>MGVEDEPLLRENPRRFVIFPIEYHDIWQMYKKAEASFWTAEDVDLSKDIQHWESLKPEERYFISHVLAFFAASDGIVNENLVERFSQEVQITEARCFYGFQIAMENIHSEMYSLLIDTY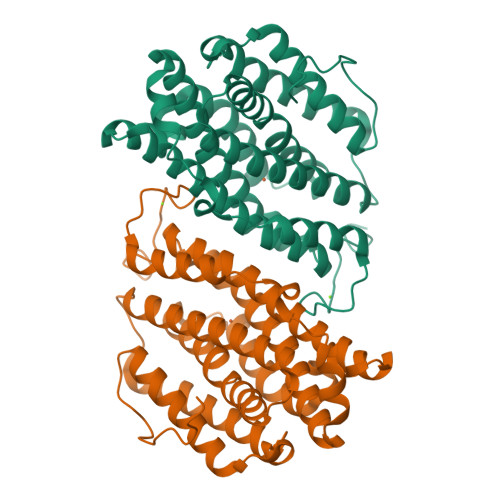IKDPKEREFLFNAIETMPCVKKKADWALRWIGDKEATYGERVVAFAAVEGIFFSGSFASIFWLKKRGLMPGLTFSNELISRDEGLHCDFACLMFKHLVHKPSEERVREIIINAVRIEQEFLTEALPVKLIGMNCTLMKQYIEFVADRLMLELGFSKVFRVENPFDFM[2x]Mammalian p97 (also called valosin-containing protein or VCP, cdc48 in yeast, and Ter94 in Drosophila) is a highly conserved AAA (ATPases associated with various cellular activities) protein with a homo-hexameric ring structure; each p97 subunit is composed of two AAA ATPase domains (D1 and D2) preceded by an N-terminal domain (N domain). VIMP, also known as selenoprotein S, is a 21 kDa ER membrane protein. VIMP, together with Derlins, is thought to contribute to the association of the p97-Ufd1-Npl4 complex with the ER membrane, forming an ER membrane-associated module in ERAD. Here we show that VIMP has an essential role in recruiting p97 to the ER membrane.

We therefore used the fragment of VIMP encompassing the minimal p97-interacting motif (residues 49−122, VIMPx) to investigate the structural basis of its interaction with p97. First, we obtained crystals of VIMPx alone, which diffracted X-rays at synchrotron to about 2 Å resolution. The structure of VIMPx consists of two long α-helices (H1 and H2) with an elbow bend at residues V70-P72 forming an elbow angle of 132.9º. The minimal p97-interacting fragment (residues 69−108) we identified is located in helix H2, immediately following the bend between the two helices, overlapping with the P-VIM (residues 78−88). Although the elbow angle (142.7°) between helices H1 and H2 in the complex (D chain in the ND1p97L198W-VIMPx) is not very different from those (132.9° and 142.2°) found in the VIMP-alone structures, the directions of the H1 helix (defined by the swing angle) in these structures are different, further supporting the notion that there is an intrinsic flexibility built into the H1-H2 joint.

> MHHHHHHQKLSARLRALRQRQLDRAAAAVEPDVVVKRQEALAAARLKMQEELNAQVEKHKEKLKQLEEEKRRQKIEMWDSM> GWL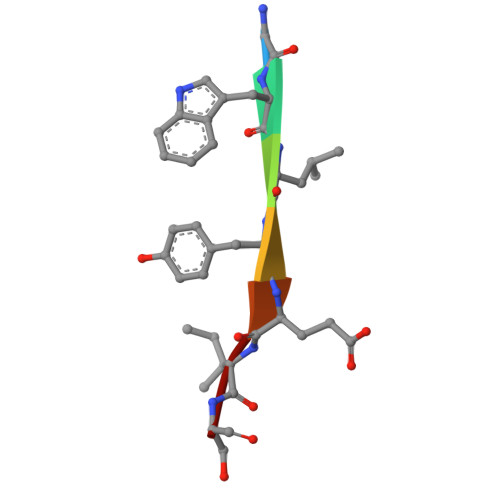YEIS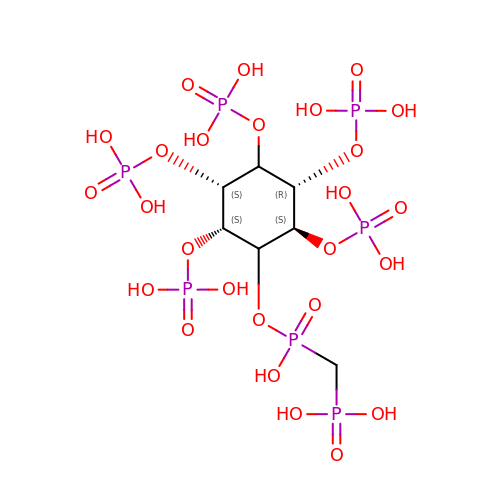[oxidanyl-[(2~{S},3~{S},5~{R},6~{S})-2,3,4,5,6-pentaphosphonooxycyclohexyl]oxy-phosphoryl]methylphosphonic acid | C7 H21 O26 P7 | IZNCMXVIYGYGJI-GESKJZQWSA-N>MNLNQLIKAAVLGGALCTACFAGAGPKGCLTPLKPVPSAEQLEWHDMEMYAFVHFTINTFTGKEWGYGDEKPELFHPSDFDADDLVRTLADAGFKGVVLTCKHHDGFCLWPTKTTLHSVAASPWKQGKGDVVKEVSRACGKYGVRFGVYLSPWDRNAASYGTPDYIRMYRQQLKELATGYGSIFLAWFDGANGGDGYYGGARERRSIDRSAYYDWKATWGELKKRQPGAVIFSDVGPDVRWVGNESGYAGYPCWATYTPVPLQAGTEPAPGTVRYRLGTEGTMDGKYWIPAEVDVSIRPGWFWHEHENSRVRTPENLLKLYFDSVGRGANLNLNVPPDRRGRIHEEDKKSLAGFRVLLDELYSRNFASGAQAESSSSWKGHGAEQVLDRKRTTYWVAAPEDKHPCVVLKLPEPAAFDVIRLAEPIQLGQRVRKFRVEVRENGQWSKWTEGASIGARVLLKGRPVTADGVRVVLEQSRAVPALCEVSLWKYPVILNAPAVNYDRNGRVTLASAENVVIRYTTDGTEPGPQSAMYRNPFFLPAGGTVKAAAEYRGRKSSVTTQIIPVPTRDWKVVAGERSAAAPELAIDGDSSTLWHTHAAQGELAPPQALEIDMGRPVNVAAVIYTPRRDSSTGTVDRYAVYLSMDGNTWGAPAAEGEFSNIRANPVPQRIDLKAPVKARYLRFVGKRVVEGSHVAVA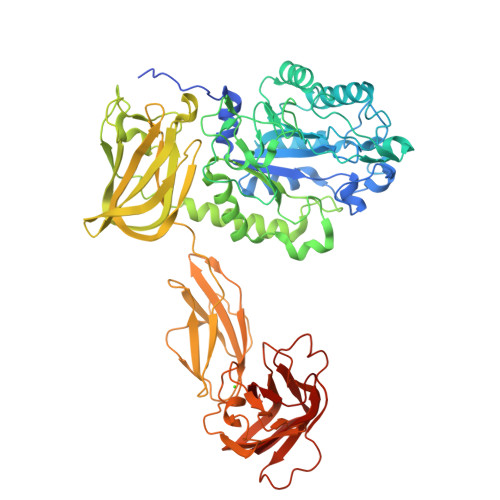ELGVLGK[2x]> MIFSVDKVRADFPVLSREVNGLPLAYLDSAASAQKPSQVIDAEAEFYRHGYAAVHRGIHTLSAQATEKMENVRKRASLFINARSAEELVFVRGTTEGIALVANSWGNSNVRAGDNIIISQMEHHANIVPWQMLCARVGAELRVIPLNPDGTLQLETLPTLFDEKTRLLAITHVSNVLGTENPLAEMITLAHQHGAKVLVDGAQAVMHHPVDVQALDCDFYVFSGHKLYGPTGIGILYVKEALLQEMPPWEGGGSMIATVSLSEGTTWTKAPWRFEAGTPNTGGIIGLGAALEYVSALGLNNIAEYEQNLMHYALSQLESVPDLTLYGPQNRLGVIAFNLGKHHAYDVGSFL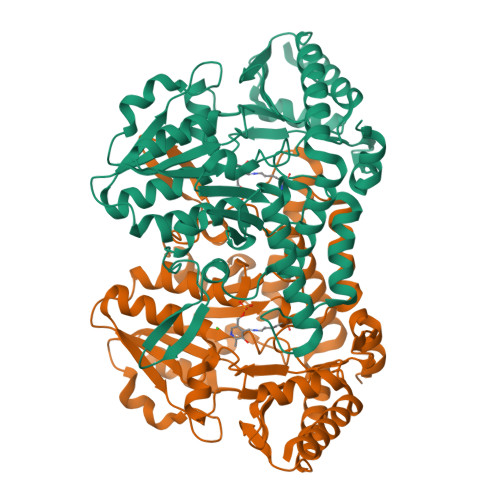DNYGIAVRTGHHCAMPLMAYYNVPAMCRASLAMYNTHEEVDRLVTGLQRIHRLLG> GSGFTSKDTYLSHFNPRDYLEKYYKFGSRHSAESQILKHLLKNLFKIFCLDGVKGDLLIDIGSGPTIYQLLSACESFKEIVVTDYSDQNLQELEKWLKKEPAAFDWSPVVTYVCDLEGNRVKGPEKEEKLRQAVKQVLKCDVTQSQPLGAVPLPPADCVLSTLCLDAACPDLPTYCRALRNLGSLLKPGGFLVIMDALKSSYYMIGEQKFSSLPLGRE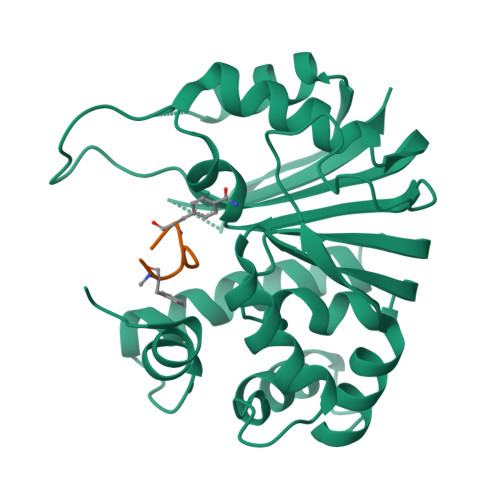AVEAAVKEAGYTIEWFEVISQSYSSTMANNEGLFSLVARKL;> GFPYKPXFC Pyruvate dehydrogenase (PDH) is a multienzyme complex that catalyzes the oxidative transformation of pyruvate to acetyl coenzyme A (CoA), CO2, and reducing equivalents in the form of NADH. The first step involves decarboxylation of pyruvate, which proceeds through formation of a covalent intermediate with the thiamine diphosphate cofactor (ThDP) in the active site of the pyruvate decarboxylase subunit (E1p; EC 1.2.4.2). E1p also catalyzes the second reaction step in which the acetyl group is transferred regiospecifically onto one of the sulfur atoms of a lipoyl moiety. The E1p enzyme from pyruvate dehydrogenase is a prototypical thiamine-dependent decarboxylase subunit from the extensive family of 2-oxo acid dehydrogenases.

We have also solved the structure of the E1p/E2p-PSBD complex with bound 2-(1-hydroxyethyl)-3-deazaThDP at 2.5 Å resolution, representing an analog of the postdecarboxylation enamine-ThDP intermediate. We prepared cocrystals of G. stearothermophilus E1p/E2p-PSBD in complex with 2-(1-hydroxyethyl)-3-deazaThDP (he-3-deazaThDP), an analog of the enamine-ThDP intermediate. The ligand he-3-deazaThDP mimics the postdecarboxylation enamine-ThDP intermediate in both structure and charge state, but with a distorted geometry. The true enamine intermediate is sp2 hybridized at C2α, but the C2α atom of our analog is sp3 hybridized. Although a racemic mixture was used in the crystallizations, the electron density map suggests that the R enantiomer was preferred in the crystal. The H128β Nɛ atom contributes to a hydrogen-bonding network involving the OA atom of he-3-deazaThDP (distance of 3.4 Å) and the cofactor's N4′ (distance 2.5 Å). We observe that the inner and outer loops are also both ordered in the he-3-deazaThDP complex structure in all four subunits of the asymmetric unit. In the crystal structure of the he-3-deazaThDP, the pocket has few apparent fixed water molecules. Our docking model suggests that by simply flipping about the Cβ-Cγ bond, the H271α Nɛ is brought away from the thiazole and orientated toward the dithiolane ring of the oxidised lipoyl group. In one of the four asymmetric unit copies of the he-deazaThDP complex, the H271α appears to have made this flip, and this is correlated with the loss of the water molecule that links the side chain to the terminal phosphate of the ThDP.

>[4x]MGVKTFQFPFAEQLEKVAEQFPTFQILNEEGEVVNEEAMPELSDEQLKELMRRMVYTRILDQRSISLNRQGRLGFYAPTAGQEASQIASHFALEKEDFILPGYRDVPQIIWHGLPLYQAFLFSRGHFHGNQIPEGVNVLPPQIIIGAQYIQAAGVALGLKMRGKKAVAITYTGDGGTSQGDFYEGINFAGAFKAPAIFVVQNNRFAISTPVEKQTVAKTLAQKAVAAGIPGIQVDGMDPLAVYAAVKAARERAINGEGPTLIETLCFRYGPHTMSGDDPTRYRSKELENEWAKKDPLVRFRKFLEAKGLWSEEEENNVIEQAKEEIKEAIKKADETPKQKVTDLISIMFEELPFNLKEQYEIYKEKESK;>MAQMTMVQAITDALRIELKNDPNVLIFGEDVGVNGGVFRATEGLQAEFGEDRVFDTPLAESGIGGLAIGLALQGFRPVPEIQFFGFVYEVMDSICGQMARIRYRTGGRYHMPITIRSPFGGGVHTPELHSDSLEGLVAQQPGLKVVIPSTPYDAKGLLISAIRDNDPVIFLEHLKLYRSFRQEVPEGEYTIPIGKADIKREGKDITIIAYGAMVHESLKAAAELEKEGISAEVVDLRTVQPLDIETIIGSVEKTGRAIVVQEAQRQAGIAANVVAEINERAILSLEAPVLRVAAPDTVYPFAQAESVWLPNFKDVIETAKKVMNF[4x];>MAFEFKLPDIGEGIHEGEIVKWFVKPGDEVNEDDVLCEVQNDKAVVEIPSPVKGKVLEILVPEGTVATVGQTLITLDAPGYENMTFKGQEQEEAKKEEKTETVSKEEKVDAVAPNAPAAEAEAGPNRRVIAMPSVRKYAREKGVDIRLVQGTGKNGRVLKEDIDAFLAGGAKPAPAAAEEKAAPAAAKPATTEGEFPETREKMSGIRRAIAKAMVHSKHTAPHVTLMDEADVTKLVAHRKKFKAIAAEKGIKLTFLPYVVKALVSALREYPVLNTSIDDETEEIIQKHYYNIGIAADTDRGLLVPVIKHADRKPIFALAQEINELAEKARDGKLTPGEMKGASCTITNIGSAGGQWFTPVINHPEVAILGIGRIAEKPIVRDGEIVAAPMLALSLSFDHRMIDGATAQKALNHIKRLLSDPELLLMEA[2x]>[2x]MTASTVAACGSDSGEIVISYYTPANEAATFTAVAQRCNAELGGRFRIEQRSLPREADAQRLQLARRLTGNDRSLDVMALDVVWTAEFAEAGWALPLSEDPAGLAEADATTNTLPGPLETAKWNGELYAAPITTNTQLLWYRADLMDEPPATWDEMLSEAARLHAQGGPSWIAVQGKQYEGLVVWFNTLLESAGGQVLSDDGQRVTLTDTPEHRAATVKALEIIKAVATAPGADPSITQTDENTARLALEQGRAALEVNWPYVLPSLLENAIKGGVGFLPLNENPALRGSINDVGTFAPTDEQFDLALNASKEVFGFARYPGVRPDEPARVTLGGLNLAVASTTRHKAEAFEAVRCLRNEENQRLTSIEGGLPAVRTSLYDDPQFQAKYPQYEIIRDQLINAAVRPATPVYQAMSTRMSATLAPISQIDPERTADELAEQVQQAIDGKGLIP

The Mycobacterium tuberculosis (Mtb) LpqY-SugABC ATP-binding cassette transporter is a recycling system that imports trehalose released during remodeling of the Mtb cell-envelope. Recent studies in mutant strains of Mtb have demonstrated that the LpqY-SugABC (Rv1235-Rv1238) ATP-binding cassette (ABC) transporter recognizes trehalose and enables the recovery and recycling of this liberated cell wall disaccharide that would otherwise be lost. The optimal conditions for the production of Mtb LpqY and mycobacterial LpqY homologs were explored extensively in Escherichia coli. This yielded LpqY from Mycobacterium thermoresistible (Mtr), which has high sequence identity (72%) to Mtb LpqY at the amino acid level. The overall architecture of Mtr LpqY is typical of substrate-binding domains of ABC transporters, consisting of two globular α/β domains joined by a hinge region, which in this instance is formed from three flexible loops.

To determine the molecular and structural basis of trehalose recognition, we solved the crystal structure of Mtr LpqY with the trehalose substrate present. The Mtr LpqY-trehalose complex crystallized in space group P412121, and the structure was determined by exploiting the anomalous signal from iodide-soaked crystals. The model containing bound iodine ions was then used as a search model to solve the structure of a native, higher-resolution, data set by molecular replacement, and the final Mtr LpqY-trehalose complex structure was refined at a resolution of 1.7 Å to an Rwork of 16.9% and Rfree of 19.4% (see Table S1 for the data collection and refinement statistics). Two Mtr LpqY protein molecules are present within the asymmetric unit. The Mtr LpqY-trehalose complex adopts a closed conformation, which is further stabilized through a central arginine residue within the hinge region (Arg404, loop 3) that forms interdomain hydrogen bonds with the carbonyl oxygen of Leu332 located on loop 2 and the carboxylate of Glu179 from domain 2 as well as being directly involved with substrate binding. The trehalose molecule was clearly defined in the electron density and resides within the acidic binding cleft formed between domains I and II and interacts with residues from both domains. In the Mtr LpqY structure, both of the glucose rings adopt a classical 4C1 chair conformation with almost equivalent dihedral angles across the glycosidic bonds (φH: 63.2°, ψH 65.4°), thus having rotational symmetry about the central glycosidic oxygen atom, mimicking the conformation of anhydrous trehalose crystallized in the absence of protein.>MEKLVQPTPLLLSLLKSAGAQKETFTMKEVLYHLGQYIMAKQLYDEKQQHIVHC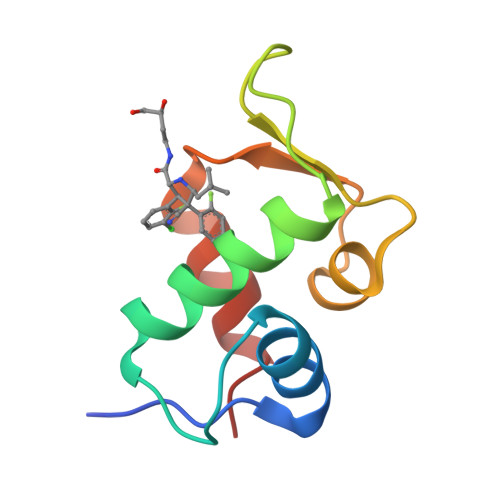SNDPLGELFGVQEFSVKEHRRIYAMISRNLVS[2x]>MSELSEIDSVAGVTIYSVDGEPKSFVYKAGFAIDADGAPNAYAPNNGGTDFTANGGDDQGGDWWGGPVDAEGYPIKQKIFDPFPGYYVSATAHFNPAYSEDSPYRYIDSNSIPFIVLPGNHSNGAKLGDVALVYNEKTGDNCYAIYGDVGPSSKIGEGSV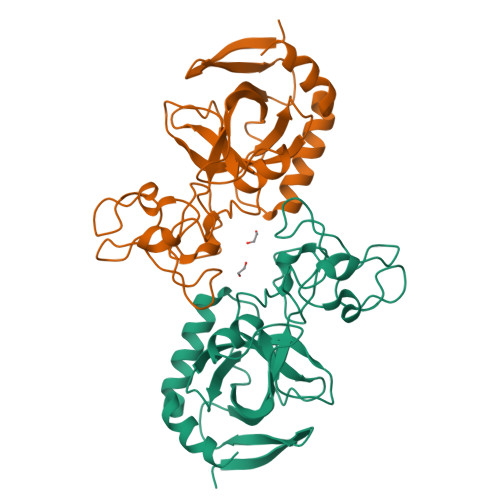RLAQALKIDDNPKAGGTESRIVVTLVFPGSVGKWETPKRWFSHANQLTKAWGGLSRLKTLSDQL[2x]> DDYLDRLPKSKKGLQGLLQDIEKRILHYKQLFFKEQNEIANGKRSMVPDNSIPICSDVTKLNFQALIDAQMRHAGKMFDVIMMDPPWQLSSSQPSRGVAIAYDSLSDEKIQNMPIQSLQQDGFIFVWAINAKYRVTIKMIENWGYKLVDEITWVKKTVNGKIAKGHGFYLQHAKESCLIGVKGDVDNGRFKKNIASDVIFSERRGQSQKPEEIYQYINQLCPNGNYLEIFARRNNLHDNWVSIGNEL;> MKKNGKSQNQPLDFTQYAKNMRKDLSNQDICLEDGALNHSYFLTK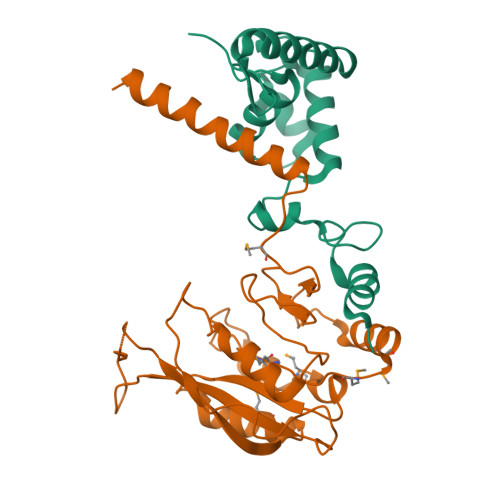KGQYWTPLNQKALQRGIELFGVGNWKEINYDEFSGKANIVELELRTCMILGINDITEYYGKKISEEEQEEIKKSNIAKGKKENKLKDNIYQKLQQMQ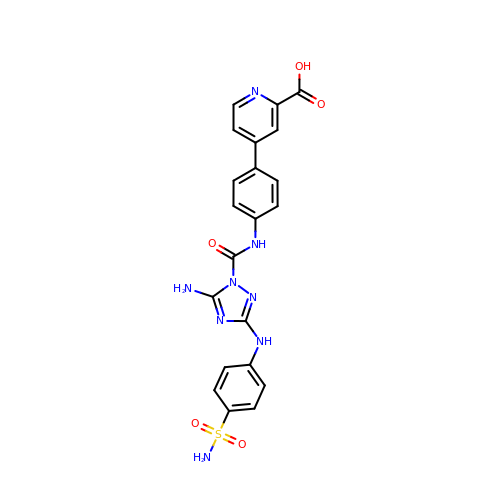4-(4-{[5-amino-3-(4-sulfamoylanilino)-1H-1,2,4-triazole-1-carbonyl]amino}phenyl)pyridine-2-carboxylic acid | C21 H18 N8 O5 S | HJIMKTSYKCAAPM-UHFFFAOYSA-N> MAKQPGLDFQSAKGGLGELKRRLLFVIGALIVFRIGSFIPIPGIDAAVLAKLLEQQRGTIIEMFNMFSGGALSRASIFALGIMPYISASIIIQLLTVVHPTLAEIKKEGESGRRKISQYTRYGTLVLAIFQSIGIATGLPNMPGMQGLVINPGFAFYFTAVVSLVTGTMFLMWLGEQITERGIGNGISIIIFAGIVAGLPPAIAHTIEQARQGDLHFLVLLLVAVLVFAVTFFVVFVERGQRRIVVNYAKRQQGRRVYAAQSTHLPLKVNMAGVIPAIFASSIILFPATIASWFGGGTGWNWLTTISLYLQPGQPLYVLLYASAIIFFCFFYTALVFN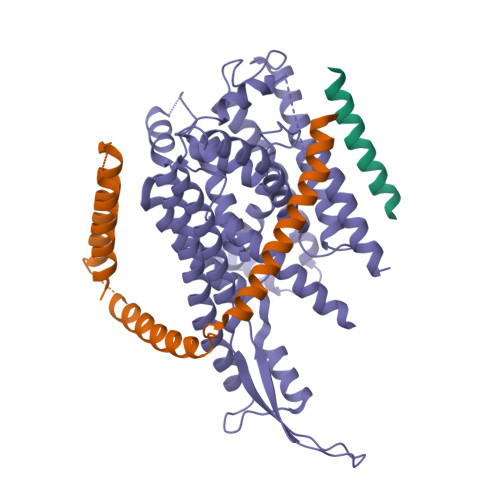PRETADNLKKSGAFVPGIRPGEQTAKYIDKVMTRLTLVGALYITFICLIPEFMRDAMKVPFYFGGTSLLIVVVVIMDFMAQVQTLMMSSQYESALKKANLKGYGR> MTQGLLAGKRFLIAGV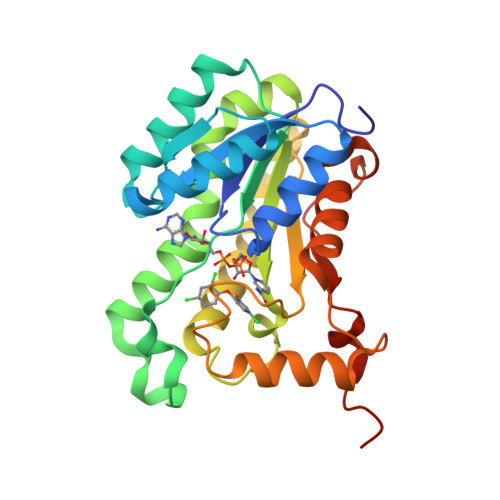ASKLSIAYGIAQALHREGAELAFTYPNEKLKKRVDEFAEQFGSKLVFPCDVAVDAEIDNAFAELAKHWDGVDGVVHSIGFAPAHTLDGDFTDVTDRDGFKIAHDISAYSFVAMARAAKPLLQARQGCLLTLTYQGSERVMPNYNVMGMAKASLEAGVRYLASSLGVDGIRVNAISAGPIRTLAASGIKSFRKMLDANEKVAPLKRNVTIEEVGNAALFLCSPWASGITGEILYVDAGFNTVGMSQSMMDDE>[3x]MSTNKVNKERTFLAVKPDGVARGLVGEIIARYEKKGFVLVGLKQLV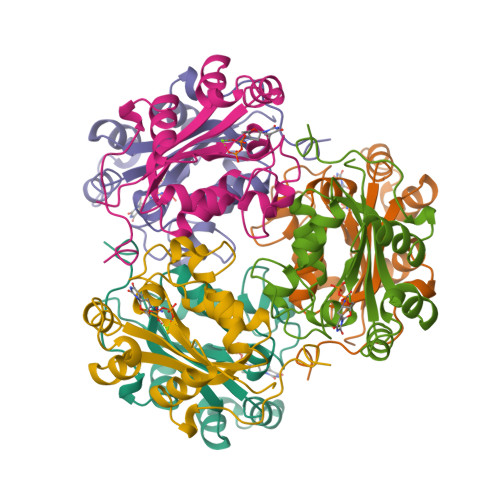PTKDLAESHYAEHKERPFFGGLVSFITSGPVVAMVFEGKGVVASARLMIGVTNPLASAPGSIRGDFGVDVGRAIIHGSDSVESANREIALWFKPEELLTEVKPNPNLYE Omniligase-1 is a broadly applicable enzyme for peptide bond formation between an activated acyl donor peptide and a non-protected acyl acceptor peptide. The enzyme is derived from an earlier subtilisin variant called peptiligase by several rounds of protein engineering aimed at increasing synthetic yields and substrate range. Mutation A225N in the S1′ pocket and F189W of the S2′ pocket increased the synthesis to hydrolysis (S/H) ratio and overall coupling efficiency, whereas the I107V mutation was added to S4 pocket to increase the reaction rate. The final omniligase variants appeared to have a very broad substrate range, coupling more than 250 peptides in a 400-member library of acyl acceptors, as indicated by a high-throughput FRET assay.

Crystals of variants containing a Trp at position 189 were only found after a long incubation time for Pre-4 (Ptl-M222P/L217H/A225N/F189W) and Pre-5 (Ptl-M222P/L217H/A225N/F189W/N218D). Mutation S218D in Pre-5 is involved in the S1′ and S2′ pockets but has no influence on the structure. The structures of Pre-4 and Pre-5 each contain three protein molecules in the asymmetric unit (molecules A-C). In both of these variants Trp189 is involved in intermolecular contacts which are different from those in Pre-1-Pre-3. In addition to the role of Phe189 in crystal formation, we observed that for both Pre-4 and Pre-5, crystallization resulted in at least one substrate binding site occupied by a peptide sequence. Variants Pre-4 and Pre-5 crystallized in crystal form C containing three protein molecules (A, B and C) in the asymmetric unit. The structures of molecules A and B are highly similar with an RMSD (root-mean square deviation) of 0.3 Å. They have oxidized cysteine and an unoccupied active site like ligases Pre-1 to Pre-3. In crystal form C the structure of molecule C is more different with RMSDs of 0.6 – 0.7 Å to molecules A and B. It has an oxidized cysteine and a bound eglin fragment (41′-46′ (SPVTLAG P5 -P1′)) that was used as a crystallization aid. In this crystal form C, we also observed a crystallization artifact; part of the loop from Ile205 to His217 of molecule C is forcibly drawn into the active site of molecule B, mimicking a peptide substrate.

>[3x]AKCVSYGVSQIKAPALHSQGYTGSNVKVAVIDSGIDSSHPDLNVAGGASFVPSETNPFQDNNSHGTHVAGTVLAVAPSASLYAVKVLGADGSGQYSWIINGIEWAIANNMDVINMSLGGPSGSAALKAAVDKAVASGVVVVAAAGNSGTSGSSSTVSYPAKYPSVIAVGAVDSSNQRAPWSSVGPELDVMAPGVSICSTLPGNKYGAHDGTCPASNHVAGAAALILSKHPNWTNTQVRSSLENTATKLGDSFYYGKGLINVEAAAQHHHHHH;> LPEGSPVTLDLRY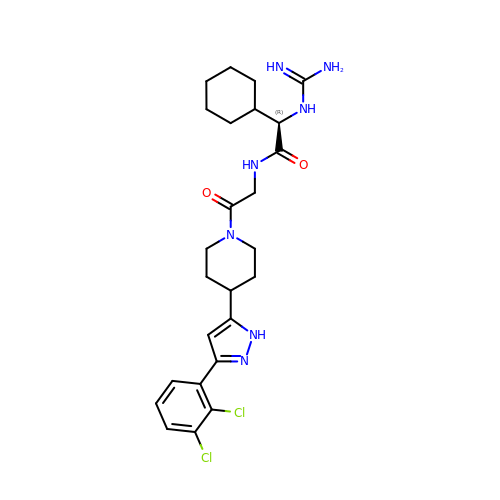2-CYCLOHEXYL-N-(2-{4-[5-(2,3-DICHLORO-PHENYL)-2H-PYRAZOL-3-YL]-PIPERIDIN-1-YL}-2-OXO-ETHYL)-2-GUANIDINO-ACETAMIDE | C25 H33 Cl2 N7 O2 | SSSXBBASYYVGCI-HSZRJFAPSA-N>[4x]SMQGPRTRARLGANEVLLVVGGFGSQQSPIDVVEKYDPKTQEWSFLPSITRKRRYVA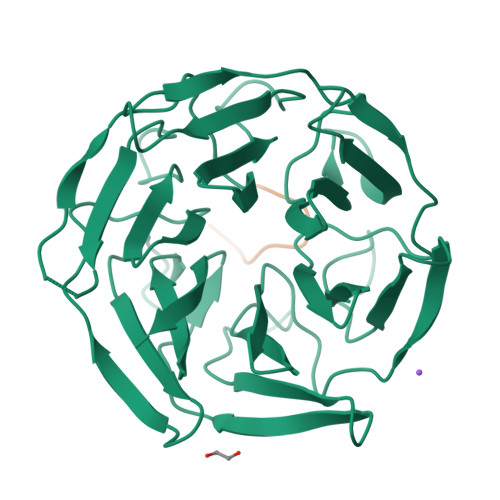SVSLHDRIYVIGGYDGRSRLSSVECLDYTADEDGVWYSVAPMNVRRGLAGATTLGDMIYVSGGFDGSRRHTSMERYDPNIDQWSMLGDMQTAREGAGLVVASGVIYCLGGYDGLNILNSVEKYDPHTGHWTNVTPMATKRSGAGVALLNDHIYVVGGFDGTAHLSSVEAYNIRTDSWTTVTSMTTPRCYVGATVLRGRLYAIAGYDGNSLLSSIECYDPIIDSWEVVTSMGTQRCDAGVCVLRE;>[4x]AYTVVGGPPGGPPVR Here we present structural convergent evolution on fusion enzymes of aldehyde dehydrogenases (ALDHs) and alcohol dehydrogenases (ADHs). We discover BdhE (bifunctional dehydrogenase E), an enzyme clade that emerged independently from the previously known AdhE family through distinct gene fusion events. AdhE and BdhE show shared enzymatic activities and non-overlapping phylogenetic distribution, suggesting common functions in different species. Intriguingly, despite distinct quaternary structures and < 30% amino acid sequence identity, both enzymes forms resemble dimeric structure units by ALDH-ADH interactions via convergently elongated loop structures.

In addition, a BN-PAGE for BdhE resulted in a single band around the molecular weight of tetramers (391.6 kDa). Therefore, BdhE was suggested to form a complex, but it is not polymer like AdhE but a stable tetramer. The results revealed that BdhE formed a ring-shaped tetramer, while AdhE formed a helical polymer, even though they were purified in the same condition. Looking into the cross-section of the BdhE tetramer’s electron density, we found that the tunnels where substrate passes were connected between ALDH and ADH domains. We found a gap in the tunnel wall formed by a BdhE dimer, which were not found in AdhE dimers. In an AdhE dimer, the linker of ALDH and ADH domains filled the gap, while the linker of BdhE formed the elongated loop (loop 2 in Fig. 4a and b) and thereby remained the gap. In BdhE, however, another BdhE dimer partially filled the gap in the tunnel wall within the tetrameric complex, suggesting that the tetrameric structure is more effective at preventing intermediate aldehydes from leaking out than the dimeric structure. Importantly, the RMSF reductions were significantly larger for BdhE tetramerization than AdhE hexamerization. The ring structure of BdhE is thus suggested to confer more rigid enzymatic activity than AdhE against environmental changes (e.g., salinity, pH, or temperature).

>[4x]MDSYQLFLDGEFVDAADGRTFTTTDPGNEQPVATVAQAGEADALRAIEAARWAFDHGEWPKMTPQERAARIYDFADHVTKLAGRLAMAESMDAGHVINLSKFWAANGAALLRNLAHYSANSFPWEEEIPYSGNVGAPGRDYIRREPIGVCVGIIPWNFPASMAFWKISHAIIMGNTIVLKPATQTPLTALIIAEAAKAAGIPKGVINVITGQGREVGNLLCTHPDVDKISFTGSTSVGNNIMKLAADSTKRVTLELGGKSANIILDDADLDAAVEGAVFGTFLHQGQVCESGTRLLVSSKIYDAFIDKLKARTEALRVGYPLSPESHLGPLVSGKQLETVEGYVKLGLEEGATLLTGGHRVEVPGISGGHYYAPTIFTDVDNRMRIAQEEIFGPVVVVIRFDSDEEAVAIANDSIYGLAGGVYSGSNARAQRVATQLRTGTVWINNYHAFGDFCPFGGYKQSGFGREMGASGLSEFVQVKRVHVSAYASVGASPAMAILSDDKKTPFVQYNAPTNIISGHGSLPAIYKEMVKLGCKRAVIMTDEGVNATGLPTLVREALDDFCVGVYDRIEQDSSLDTVDAAAAYARECGADAIVSVGGGSVIDTSKAVCVVLKNGGKCNDHMAMLRLQEPQTPHIAIPTTSGTGSEVTNVAVIKNKAVGRKVYILDPHIVPNSTILDPRFTLGLPHRMTVTTALDAMTHSIEALTSTRSQPICDGQALQAIRLISENLPRVVAKPHDEAARANLQLAATMAGWAFNVAQVGLAHAMAHTLGAIHDIPHGLACGIMLPRVMRFNVDHAGHKLALAAQALGVQTTGMDAREAGLAAAQAVEALMQSVDHPRYLSDLGVPRDNLSNLAAHAMGDAAIMFNARPVKGPQEVMAVYEEAY>MSYTKEQLMLAFSYMSYYGITHTGSAKKNAELILKKMKEALKTWKPFQEDDWEVVWGPAVY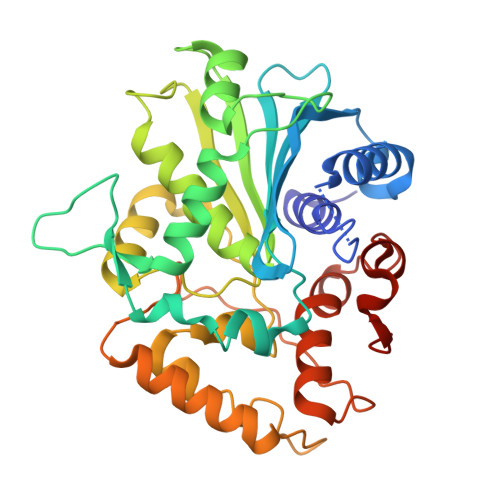TMPFTIFNDAMMYVIQKKGAEGEYVIAIRGTNPVSISDWLFNDFMVSAMKKWPYASVEGRILKISESTSYGLKTLQKLKPKSHIPGENKTILQFLNEKIGPEGKAKICVTGHSKGGALSSTLALWLKDIQGVKLSQNIDISTIPFAGPTAGNADFADYFDDCLGDQCTRIANSLDIVPYAWNTNSLKKLKSIYISEQASVKPLLYQRALIRAMIAETKGKKYKQIKAETPPLEGNINPILIEYLVQAAYQHVVGYPELMGMMDDIPLTDIFEDAIAGLLHHHHHH[2x]> MAHHHHHHVDDDDKMSASKEIKSFLWTQSLRRELSGYCSNIKLQVVKDAQALLHGLDFSEVSNVQRLMRKERRDDNDLKRLRDLNQAVNNLVELKSTQQKSILRVGTLTSDDLLILAADLEKLKSKVIRTERPLSAGVYMGNLSSQQLDQRRALLNMIGMSGGNQGARAGRDGVVRVWDVKNAELLSNQFGTMPSLTLACLTKQGQVDLNDAVQALTDLGLIYTAKYPNTSDLDRLTQSHPILNMIDTKKSSLNISGYNFSLGAAVKAGAC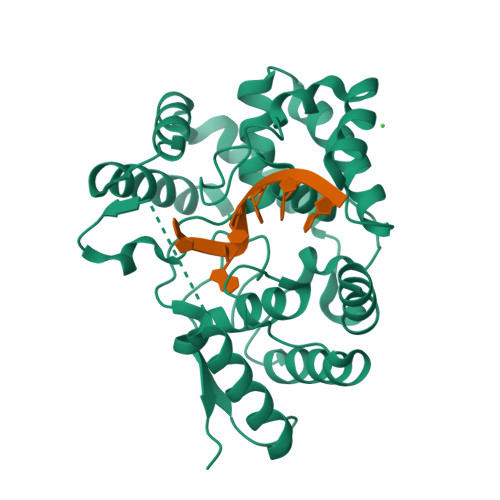MLDGGNMLETIKVSPQTMDGILKSILKVKKALGMFISDTPGERNPYENILYKICLSGDGWPYIASRTSITGRAWENTVVDLES> MSDKIIHLTDD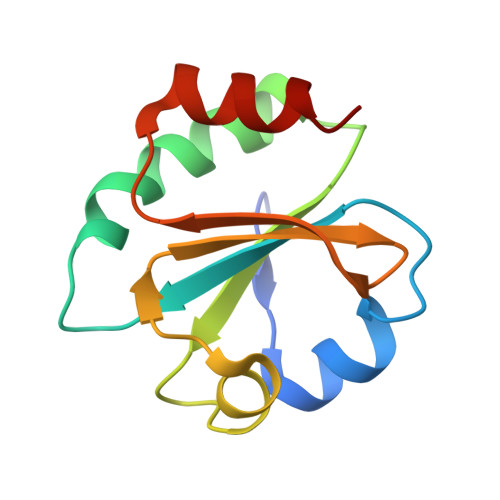SFDTDVLKADGAILVDFWAEWCGPCKMIAPILDEIADEYQGKLTVAKLNIDQNPGTAPKYGIRGIPTLLLFKNGEVAATKVGALSKGQLKEFLDANLA> GSMVEATAQETDRPRFSFSIAAREGKARTGTIEMKRGVIRTPAFMPVGTAATVKALKPETVRATGADIILGNTYHLMLRPGAERIAKLGGLHSFMGWDRPILTDSGGYQVMSLSSLTKQSEEGVTFKSHLDGSRHMLSPERSIEIQHLLGSDIVMAFDECTPYPATPSRAASSMERSMRWAKRSRDAFDSRKEQAENAALFGIQQGSVFENLRQQSADALAEIGFDGYAVGGLAVGEGQDEMFRVLDFSVPMLPDDKPHYLM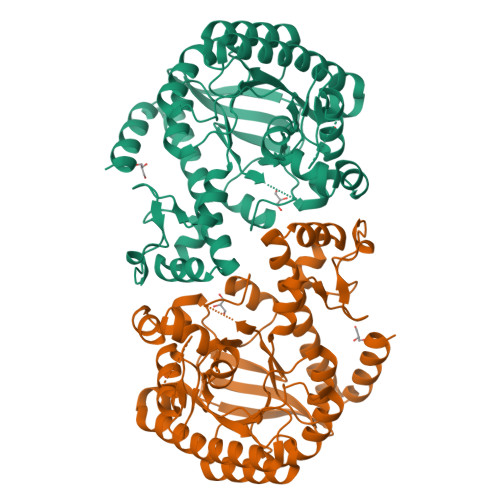GVGKPDDIVGAVERGIDMFDCVLPTRSGRNGQAFTWDGPINIRNARFSEDLKPLDSECHCAVCQKWSRAYIHALIRAGEILGAMLMTEHNIAFYQQLMQKIRDSISEGRFSQFAQDFRARYFARNS>[2x]MVLYFIGLGLYDERDITVKGLEIAKKCDYVFAEFYTSMMAGTTLGRIQKLIGKEIRVLSREDVELNFENIVLPLAKENDVAFLTPGDPLVATTHAELRIRAKRAGVESYVIHAPSIYSAVGITGLHIYKFGKSATVAYPEGNWFPTSYYDVIKENAERGLHTLLFLDIKAEKRMYMTANEAMELLLKVEDMKKGGVFTDDTLVVVLARAGSLNPTIR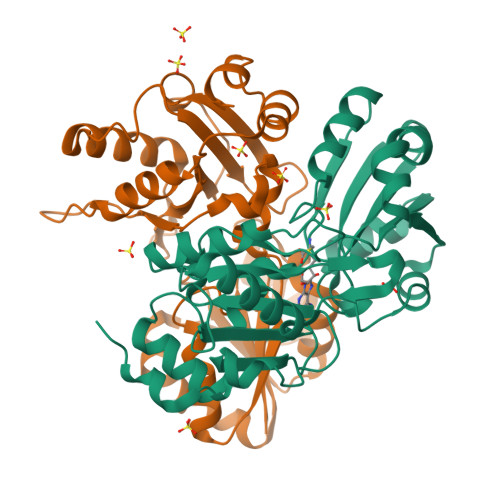AGYVKDLIREDFGDPPHILIVPGKLHIVEAEYLVEIAGAPREILRVNV Lipin/Pah phosphatidic acid phosphatases (PAPs) are Mg2+-dependent enzymes that catalyze the dephosphorylation of phosphatidic acid (PA) to produce diacylglycerol. pmcLipin/Pah phosphatidic acid phosphatases (PAPs) are magnesium-dependent enzymes that are evolutionarily conserved from yeast to humans. They catalyze the penultimate step of triacylglycerol synthesis, through the conversion of phosphatidic acid (PA) to diacylglycerol (DAG). Structurally, all lipin/Pah PAPs contain highly conserved N-Lip and C-Lip regions that combine to form two domains: an immunoglobulin-like (Ig-like) domain and a HAD-like catalytic domain. The remainder of the C-Lip adopts a Rossmann-fold, forming the haloacid dehalogenase-like (HAD-like) domain and harbors a conserved catalytic motif DxDxT, where the first Asp coordinates a Mg2+ ion that increases its nucleophilicity, and the second Asp participates in acid/base catalysis.

Structure 1 was determined using a Δhelix-His construct that lacked the N-terminal helix but included a C-terminal His-tag. The Δhelix-His structure represented an inactive state due to covalent modification of Cys276 by cacodylate, which was present in the crystallization solution. Cacodylate modification of Cys276, which lies below the nucleophilic Asp of the DxDxT motif, induced a major rearrangement of active site loops and residues, including an Asn residue (N268) that binds Mg2+, the adjacent Arg residue (R269) we implicate in PA recognition below, and an Asp residue (D272) that is mutated to His or Asn in rhabdomyolysis, which formed a hydrogen bond with a Mg2+ bound water in other active states of catalysis. In sharp contrast, in the Δhelix-His structure (Structure 1), cap region 2 formed an upward facing alpha helix that was continuous with the prior helix and would be perpendicular to the membrane interface. This unique conformation was formed through crystal contacts, with the continuous alpha helix packing into the active site of an adjacent molecule. We thus consider this conformation of cap region 2 to be an artifact of crystallization and represent a catalytically incompetent state. However, it does highlight the flexibility of cap region 2, which may be important for the regulation of lipin/Pah PAP activity.

>[2x]SMFSGVVDIIVVRQPDDSLKSMPFHIRFGTLKVLDNQNINIQITVNDKKIEDVFMLMLPEGACYFPELNAKNEIQKKLRPSSAILKKFNLKNGYNKIQFIAESDLQGKQLIEGKIYLYNYDTKLVISDVDGTVTKSDVKGHISTIIGKEWTHDDIAELYTNIQKNGYKMVYLSSRPLYFYNYTQGYLKGIIQNGFTMPDGPILLSPDQIISSLNREVVYKKADEFKGALLKDLRRVFPEEVNPIFAGFGNRDTDATACLYAGVIIDNIFIINEQSQVEILGKQEKSSYKKINEKIQELFPRLPAAALEHHHHH>[4x]MLSGLNHLTLAVSQLAPSVAFYQQLLGMTLHARWDSGAYLSCGDLWLCLSLDPQRRVTPPEESDYTHYAFSISEADFAS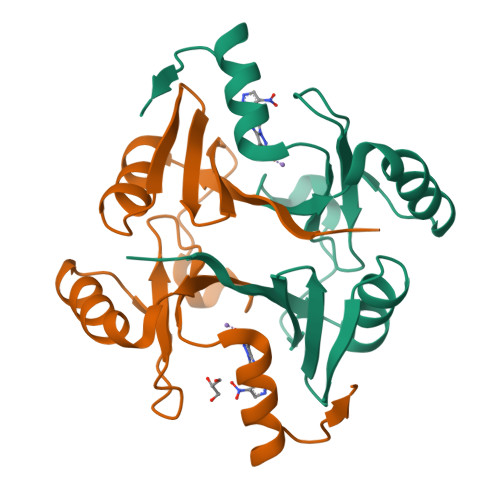FAARLEAAGVAVWKLNRSEGASHYFLDPDGHKLELHVGSLAQRLAACREQPYKGMVFFEQHHHHHH> DNGGYVPAVVIGTGYGAAVSALRLGEAGVQTLMLEMGQLWNQPGPDGNIFCGMLNPDKRSSWFKNRTEAPLGSFLWLDVVNRNIDPYAGVLDRVNYDQMSVYVGRGVGGGSLVNGGMAVEPKRSYFEEIL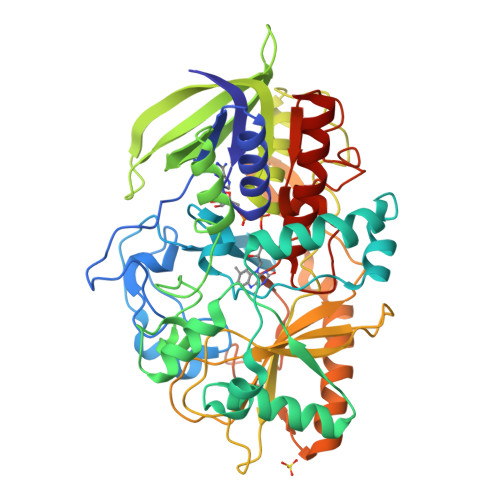PRVDSSEMYDRYFPRANSMLRVNHIDTKWFEDTEWYKFARVSREQAGKAGLGTVFVPNVYDFGYMQREAAGEVPKSALATEVIYGNNHGKQSLDKTYLAAALGTGKVTIQTLHQVKTIRQTKDGGYALTVEQKDTDGKLLATKEISCRYLFLGAGSLGSTELLVRARDTGTLPNLNSEVGAGWGPNGNIMTARANHMWNPTGAHQSSIPALGIDAWDNSDSSVFAEIAPMPAGLETWVSLYLAITKNPQRGTFVYDAATDRAKLNWTRDQNAPAVNAAKALFDRINKANGTIYRYDLFGTQLKAFADDFCYHPLGGCVLGKATDDYGRVAGYKNLYVTDGSLIPGSVGVLPFVTITALAERNVERIIKQDVTAS5'-CHLORO-N-{(3S)-1-[(1S)-1-METHYL-2-MORPHOLIN-4-YL-2-OXOETHYL]-2-OXOPYRROLIDIN-3-YL}-2,2'-BITHIOPHENE-5-SULFONAMIDE 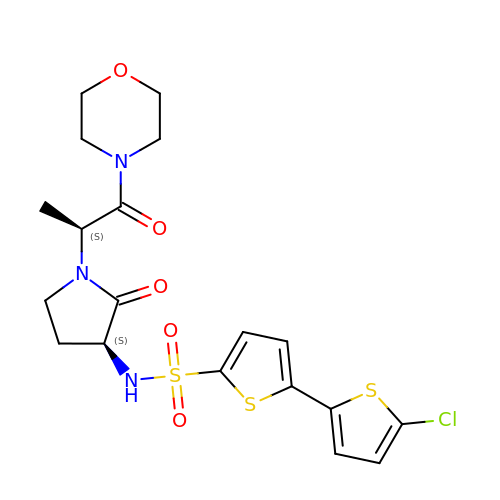| C19 H22 Cl N3 O5 S3 | NAHOZYBRUMVDSR-STQMWFEESA-N In N. gonorrhoeae, the best characterized and most clinically important multidrug efflux system that mediates multidrug resistance (MDR) is the multiple transferrable resistance (Mtr)CDE tripartite efflux pump. MtrD works in conjunction with the MtrC periplasmic membrane fusion protein and MtrE outer membrane channel to actively export antimicrobials out of bacterial cells. The cryo-EM structure of MtrDCR103 revealed that this multidrug efflux pump adopts the overall fold of hydrophobe-amphiphile efflux (HAE)-RND-type proteins and forms a homotrimer. Each protomer contains 12 transmembrane helices (TM1 to TM12) and a large periplasmic domain, which can be divided into six subdomains (PN1, PN2, PC1, PC2, DN, and DC).

The reconstituted sample led to a cryo-EM map at a nominal resolution of 3.02 Å, allowing us to obtain a structural model of this pump. Interestingly, the cryo-EM structure of MtrDCR103 indicates that this multidrug efflux pump forms an asymmetric trimer of which the three protomers are distinct and display different conformational states. Like the structure of asymmetric AcrB, the conformations of the three MtrDCR103 protomers can be classified as the “access,” “binding,” and “extrusion” forms. Unexpectedly, an extra density was found within the distal drug-binding site of the binding protomer of MtrDCR103, indicating that our structure of MtrDCR103 is bound by a fortuitous ligand. The shape of this extra density is compatible with a hydrolyzed, decarboxylated ampicillin (Amp) antibiotic with its four-member β-lactam ring open. This is not surprising, as we supplemented with 100 μg/ml ampicillin in Luria-Bertani (LB) broth to grow E. coli BL21(DE3)ΔacrB/pET15bΩmtrDCR103 cells for overproducing the MtrDCR103 protein. Within 4.5 Å of this bound deactivated Amp, there are five hydrophobic residues, including F136, I139, F176, V607, and F610, which provide hydrophobic interaction at this distal site to stabilize substrate binding. In addition, N135, S275, and T277 are involved and perform an electrostatic interaction to anchor this inactive drug. Interestingly, a positively charged residue R174 is found within the vicinity of this Amp binding site. The cryo-EM structure of the MtrDCR103-Amp complex indicates that at least 17 phosphatidylethanolamine (PE) lipids are anchored within the transmembrane domain.

>[3x]MAKFFIDRPIFAWVISIFIIAAGIFGIKSLPVSQYPSVAAPTITLHAIYPGASAQVMEGSVLSVIERNMNGVEGLDYMSTSADSSGSGSVSLTFTPDTDENLAQVEVQNKLSEVLSTLPATVQQYGVTVSKARSNFLMIVMLSSDVQSTEEMNDYAQRNVVPELQRIEGVGQVRLFGAQRAMRIWVDPKKLQNYNLSFADVGSALSAQNIQISAGSIGSLPAVRGQTVTATVTAQGQLGTAEEFGNVILRANTDGSNIYLKDVAKVGLGMEDYSSSTRLNGVNTTGMAVMLSNSGNAMATAKAVKERLAVLEKYFPQGMSWKTPYDTSKFVEISIEKVIHTLIEAMVLVFVVMYLFLQNIRYTLIPTIVVPISLLGGFAFISYMGMSINVLTMFAMILVIGIVVDDAIVVVENVERIMAGEGLPPKEATKKAMGQISGAVIGITAVLISVFVPLAMFSGAAGNIYKQFALTMASSIAFSAFLALTLTPALCATMLKTIPKGHHEEKKGFFGWFNKKFDSWTHGYEGRVAKVLRKTFRMMVVYIGLAVVGVFLFMRLPTSFLPTEDQGFVMVSVQLPAGATKERTDATLAQVTQLAKSIPEIENIITVSGFSFSGSGQNMAMGFAILKDWNERTASGSDAVAVAGKLTGMMMGTLKDGFGIAVVPPPILELGNGSGLSINLQDRNNTGHTALLAKRNELIQKMRASGLFDPSTVRAGGLEDSPQLKIDINRAAAAAQGVSFADIRTALASALSSSYVSDFPNQGRLQRVMVQADGDARMQPADILNLTVPNSSGIAVPLSSIATVSWQMGTEQSVRFNGYPAMELSGSPATGVSTGQAMEAVQKMVDELGSGYSLEWGGQSREEAKGGSQTIALYALAAVAVFLVLAALYESWSIPLAVLLVMPLGLAGAAAGVTGRNLFEGLLGSVPSFANDIYFQVGFVTVMGLSAKNAILIIEFAKDLQAQGKSAVEAALEAARLRFRPIIMTSFAFILGVVPLYIAGGASSASQRAIGTTVFWGMLIGTLLSVFLVPLFYVVVRKFFKETAHEHEM> MLRGSILSAQSTGAFSCGAAAVMPSLRSANSLHGSFAASAAFSSPISTTTSCLDVSQNQERGLSTEATGEGESEDDPTYLRGIKTQSGLRNSDGDEEPPDRRKAYEFEPGGRGRGGGGGGGGAPFQRRPADAAAAGTDMLELVATARELFTRNVDSGSGGGGAGGGGGGGGGVGPLPPLPRELREALYGHRWDR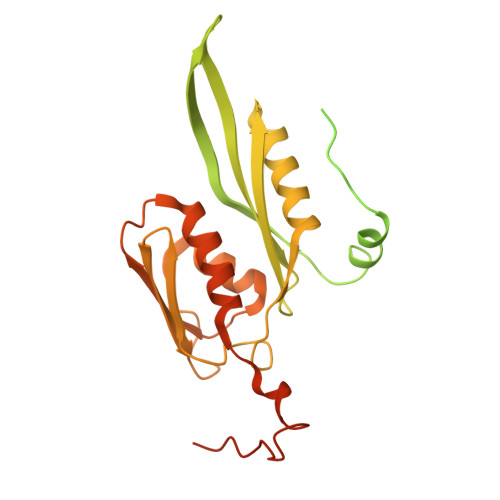VIVDVRRTHTPVRGRGKREEYTAMVATGNMRGVFGLGIGVAESAQLATARAHLDSLSRLAAVPLYRGHTLYTHVDHTFHRLSIRMMPRPAGWGLRCPDLLYELCGLVGLRDVSIRVRGQRGSRFFVAQCFQEALQKQTTPHDGVEATGMYIREVFRGGPGGRLPCGLRRGVDVM> Q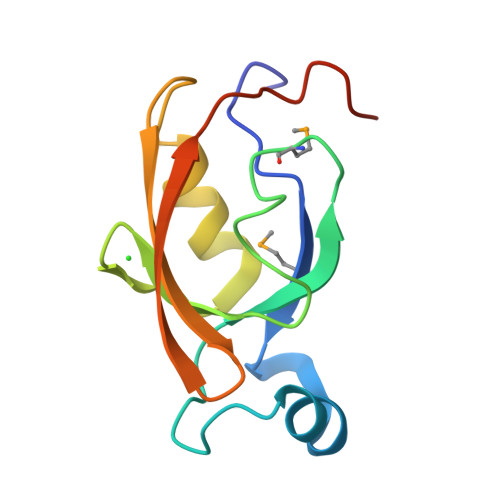VERPALGISMAGLSNLPSDVISKLKIPSNVTNGIVVASIQSGMPAQGKLKKYDVITKVDDKEVASPSDLQSLLYGHQVGDSITVTFYRGENKQTITIKLTKTSKDLAENLYFQ>MRGSHHHHHHGSMDEFEMIKRNTSEIISEEELREVLKKDEKSAGIGFEPSGKIHLGHYLQIKKMIDLQNAGFDIIIWLADLGAYLNQKGELDEIRKIGDYNKKVFEAMGLKAKYVYGSEHNLDKDYTLNVYRLALKTTLKRARRSMELIAREDENPKVAEVIYPIMQVNAIHYNGVDVAVGGMEQRKIHMLARELLPKKVVCIHNPVLTGLDGEGKMSSSKGNFIAVDDSPEEIRAKIKKAYCPAGVVEGNPIMEIAKYFLEYPLTIKRPEKFGGDLTVNSYEELESLFKNKELHPMRLKNAVAEE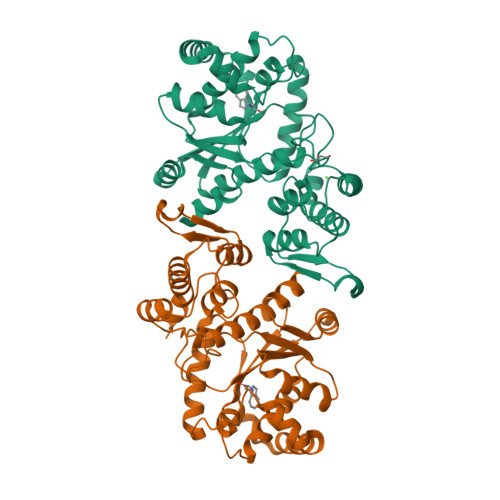LIKILEPIRKRL[4x]>[2x]MERVLIVNADDFGLSKGQNYGIIEACRNGVVTSTTALVNGAAIDHAAQLGRSTPELAVGMHFVLTLGEPLSAMPGLTRDGRLGKWIWQQAEEDSLPLEEIAHELACQYHRFVELFGHEPTHIDSHHHVHMFAQIYPIVAAFAREKGIALRIDRQVAAQSGLDQQAARSSAGFSSEFYGEAVSEELFLQTLDASIARGERSLEVMCHPAYVDRIIMGSAYCYPRLDELDVLTAASLKAAVADRGYRLGTYRDVLE

The chitobiose (chb) operon is involved in the synthesis of chitooligosaccharide and is comprised of a BCARFG gene cluster. ChbG encodes a chitooligosaccharide deacetylase (CDA) which catalyzes the removal of one acetyl group from N,N’-diacetylchitobiose. It is considered a novel type of CDA due to its lack of sequence homology. ChbG is a unique COD that is conserved in bacteria to mammalian genomes.

Thereafter, the purified protein was crystallized, and the 1.83 Å crystal structure was solved using the molecular replacement phasing method and refined to Rwork = 20.24 % and Rfree = 25.02 %. Two molecules (A and B) were found in the crystallographic asymmetric unit. The kpChbG crystal structure showed the typical fold of the YdjC family and contained an unbalanced α/β barrel fold consisting of eleven α-helices (α1–α11) and seven β-sheets (β1–β7). An acetate molecule and metal ion were found in the putative active site of kpChbG. Clear metal ion density coordinated by D11, H61, and H125 was detected at the putative active site of kpChbG. The metal ion was identified as Zn2+ by inductively coupled plasma mass spectrometry (ICP-MS)23 with a detected concentration of 701.7 ppb (µg/kg) in around 30 µM of ChbG protein. The acetate ion was coordinated by L13, L66, S217, and R223. Residues D10 and H206 might be responsible for kpChbG deacetylation activity by working as a general base and acid, respectively, since they were also localized at the putative active site. The theoretical molecular weight of monomeric kpChbG, including the C-terminal his-tag is 30.2 kDa. Multi-angle light scattering (MALS) showed that the absolute molecular mass of kpChbG in solution was 64.9 kDa (2.1 % fitting error), which confirmed that kpChbG is a dimer in solution. Since kpChbG had the shortest α3/β3 connecting loop and the α9 helix was localized far from the α3/β3 connecting loop, the tentative active site of kpChbG showed an open conformation with a wider, deeper groove than observed in the other two homologs.> KHQVFPSFHGADVRKTILSHILESFRRKGIDPFIDNNIERSKSIGHELKEAIKGSKIAIVLLSKNYASSSWCLDELAEIMKCRELLGQIVMTIFYEVDPTDIKKQTGEFGKAFTKTCKGKTKEYVERWRKALEDVATIAGYHSH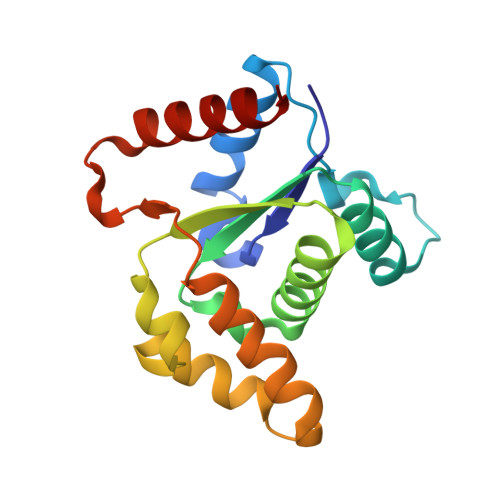KWRNEADMIEKIATDVSNMLN~{N}-[1-[(3~{R})-1-[4-(dimethylamino)but-2-enoyl]azepan-3-yl]-7-methyl-benzimidazol-2-yl]-2-methyl-pyridine-4-carboxamide 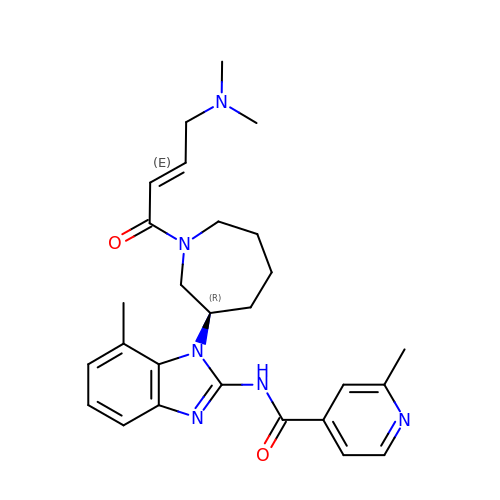| C27 H34 N6 O2 | SKLAQDNYYXAFGK-QWDXWUACSA-N[HYDROXY(3-PHENYLPROPYL)AMINO]METHANOL | C10 H15 N O2 | 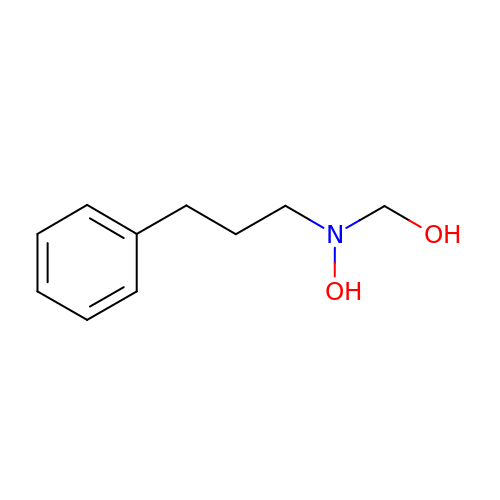GELOPWXSYZDPJT-UHFFFAOYSA-N> VTSYTLNEVVPLKD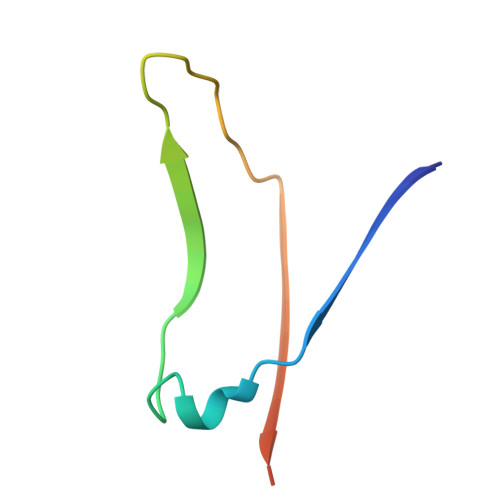VVPEWVRIGFSATTGAEFAAQEVHSWSFNSQLGHTSKS> 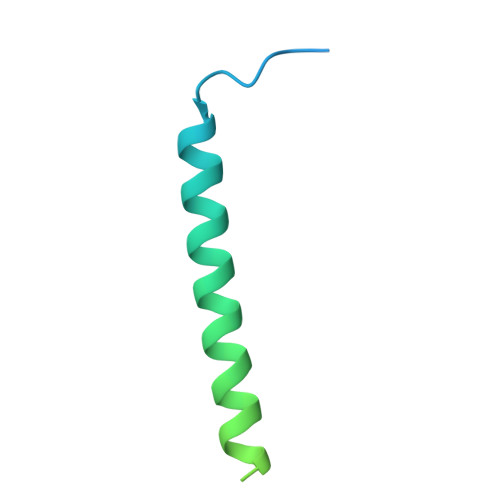GPGSNSKNPVPVKKEAKLSEAELHDKIAALEEEKAELFEKLDKVEEEHKKVEEEHKKDHEKLEKKSEDVERHYLRQLDQEYKEQQERQKNLEELERQSQREVEK> GDLADRFAELERRYDARLGVYVPATGTTAAIEYRADERFAFCSTFKAPLVAAVLHQNPLTHLDKLITYTSDDIRSISPVAQQHVQTGMTIGQLCDAAIRYSDS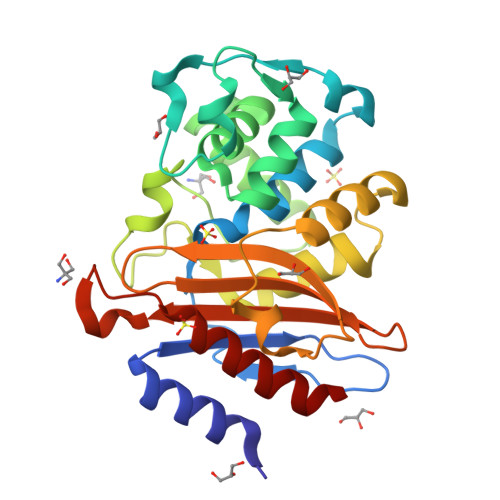TAANLLLADLGGPGGGTAAFTGYLRSLGDTVSRLDAEEPELNRDPPGDERDTTTPHAIALVLQQLVLGNALPPDKRALLTDWMARNTTGAKRIRAGFPADWKVIDKTGTGDYGRANDIAVVWSPTGVPYVVAVMSDRAGGGYDAEPREALLAEAATCVAGVLA>[4x]GSSHHHHHHSSGENLYFQGHMTCPFADPAALYSRQDTTSGQSPLAAYEVDDSTGYLTSDVGGPIQDQTSLKAGIRGPTLLEDFMFRQKIQHFDHERVPERAVHARGAGAHGTFTSYADWSNITAASFLNATGKQTPVFVRFSTVAGSRGSADTARDVHGFATRFYTDEGNFDIVGANIPVFFIQDAIQFPDLIHSVKPRPDNEIPQAATAHDSAWDFFSQQPSTMHTLFWAMSGH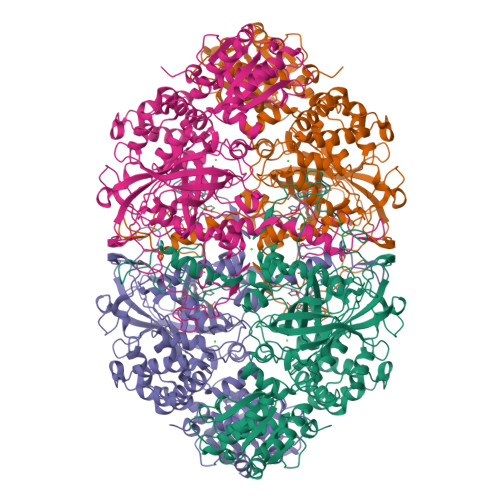GIPRSYRHMDGFGVHTFRFVKDDGSSKLIKWHFKSRQGKASLVWEEAQVLSGKNADFHRQDLWDAIESGNGPEWDVCVQIVDESQAQAFGFDLLDPTKIIPEEYAPLTKLGLLKLDRNPTNYFAETEQVMFQPGHIVRGIDFTEDPLLQGRLFSYLDTQLNRNGGPNFEQLPINMPRVPIHNNNRDGAGQMFIHRNKYPYTPNTLNSGYPRQANQNAGRGFFTAPGRTASGALVREVSPTFNDHWSQPRLFFNSLTPVEQQFLVNAMRFEISLVKSEEVKKNVLTQLNRVSHDVAVRVAAAIGLGAPDADDTYYHNNKTAGVSIVGSGPLPTIKTLRVGILATTSESSALDQAAQLRTRLEKDGLVVTVVAETLREGVDQTYSTADATGFDGVVVVDGAAALFASTASSPLFPTGRPLQIFVDAYRWGKPVGVCGGKSSEVLDAADVPEDGDGVYSEESVDMFVEEFEKGLATFRFTDRFALDS>[4x]HMSFSHVCQVGDPVLRGVAAPVERAQLGGPELQRLTQRLVQVMRRRRCVGLSAPQLGVPRQVLALELPEALCRECPPRQRALRQMEPFPLRVFVNPSLRVLDSRLVTFPEGC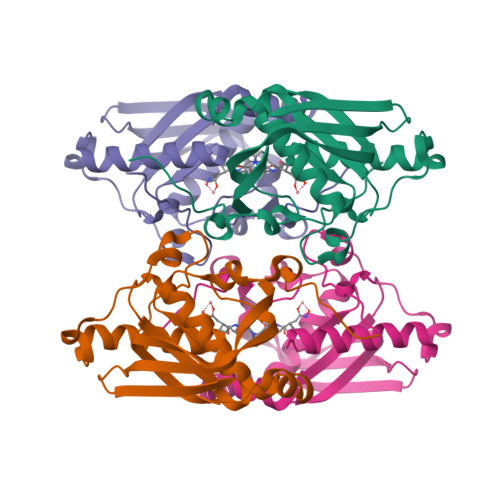ESVAGFLACVPRFQAVQISGLDPNGEQVVWQASGWAARIIQHEMDHLQGCLFIDKMDSRTFTNVYWMKVND One broad family of bacterial polymorphic toxins gathers multidomain proteins with a modular organization, comprising a C-terminal toxin domain fused to a N-terminal domain that adapts to the delivery apparatus. We recently described and characterized Tre23, a toxin domain fused to a T6SS-associated Rhs protein in Photorhabdus laumondii, Rhs1. Recently, we characterized a new toxin domain associated to a Rhs element in Photorhabdus laumondii. This Rhs1 toxin, encoded by the plu0353 gene, is delivered by the T6SS, through interactions with VgrG (Plu0355) and the Eag chaperone (EagR, Plu0354). Tre23 inhibits protein synthesis through ADP-ribosylation of helix 44 of the ribosomal 23 S RNA, hence preventing protein elongation by blocking the GTPase-associated center.

The Rhs1-EagR complex was purified from E. coli overproducing FLAG-tagged Rhs1 and Strep-tagged EagR by Streptag affinity followed by size-exclusion chromatography. In order to prevent Rhs1 autocleavage, a catalytic-null mutant, D1338N (see below), was used. We then performed an unmasked refinement to 3.72 Å followed by a local refinement on Rhs1Shell and obtained a resolution of 3.17 Å for this region. In the high-resolution cryo-EM densities obtained, we could build de novo an atomic model of Rhs1Shell from amino acids (aa) 272 to 1357. Rhs1Shell is composed of a continuous strip of antiparallel sheets (residues 420-1262) defining a hollow barrel, which is closed on each side by two plugs (residues 272–420 and 1263-1357 respectively). The C-terminal plug is deeply embedded in the Rhs1 β-barrel and tightly closes one side of the barrel. The N-terminal plug caps the other side of the Rhs1 β-barrel but remains at the exterior. It is composed of an Immunoglobulin-like (Ig-like) domain (336–421) preceded by a small extended domain sealing it to the Rhs1 β-barrel. The β-barrel and the two plugs define a central cavity of ~28,000 Å3 in volume. In this cavity, densities are visible but not well resolved, confirming that the C-terminal toxin domain is encapsulated into the Rhs1 β-barrel but suggesting that it is highly flexible and/or partially unfolded.

> MSLGDEIVTRIARVGARHAVHVSPPQGSPGPAAAREGDPIKHASFLGALAGAITGALIGAAVFAAASALVGLTILTGGLATVAVIALGTAATFALGDVISAASSAVTNMVDSIGPPSGTLTSGSPNVFIEGQPAARATTDIAVCSKHPAPPLIAQGSETVLINGSPAARVDDKLACGATIKSGAKTVFIGSGQGTYLAVADEFSAWERAILIAVEFLVPPSRGALKGLGKLFTKPGQGIQGVLKGAKAGAKKAKALLSNRISCAKKAFRETEGAKRYREATKKFFTGDPIDVTTGQLFDQRTDITLGQTLPLVFLRSWVPEEQGLLGPGWTDSFSECALATGDRVEIRTTEGASLYFALPAAYTHSVNPDHPDFTLSRGEQGYILRHRDSPVSKYFTLPHPSSASKEAPRRWLLTEHRDVYDNRLRFIYNKHCQLTQVLHSDGPELTLLYNLRGQLTEIRRTDERLQEVMARYHYHDNGRLAEADSTQNFHLYYEYNAQGLISRWSDGDQTWVDYRYDKQGRCTDSVGAGGFYPVHLDYAPGITRSTTPQGHTTTGHYNDQQLITEIHTPCGGVTRYEYDRWGNLVRQILPEGETLTLTYLADTGRVTSLTEATGAVWQYSYEADSLQLTGMTDPLQRTWLPQYDEQGQPAGFIAPDGRKTTLTRNAFGLVTSETDPDGNSRTQEYDKHQRLVRVLDEENRTVSLGYDSQDRLRSLTAAGALWRWRYDRHHRVAVSDRPDNQLEHFTHDRHGNLTCWTDARGVKWQVEYGPFDLPVARRDGEGHRWQYRYDADTLQLTQVINPQGETYSYTLDADGRVITEQDYAGTQWHYRYDRSGNCIEKRDGEENVTRYDYDAARRLTTLHTPEGPTRYHYDSVGRLLTVDSPDSTLHFEYDGQDRIVREIQPHGEIQRHYPDNRTAERQLLTGETAPVTGPARFSGQTHPGRWQSRREVNRVGELITLTLAGQAPLTIERDDAGRDTGRYVDGGFILRQQYSLMGQLTAQRAGRNPYFFRPAEPDEIEGPAYAGVARRYEYDTALNLTAASDDGQQVNYLLNGNGQVISVGEGRTLREHYQYDETGYPSRRFDGVQEIMGETLYQEGHRLNWVGSHRFVYDRAGRMQEKQFLAEGCRLALTKYRWNSQNQLTGLITPDGIPWEYRYDAFGRRTEKRCIQSGKLTTYLWDGNVPAEIREYQHGRLKMIRHLVFDGWELVAQQTQAFTLNLDNRVELMAGEVQTQYAVSAPTGEPLALFDPAGKRVWRRPKQSLYGLRLGGYGENPQLDPGLRFAGQLFDEESGLFYNRFRYYLPEATCYLSPDPTGLWGGENTYRYVQNPTKFINPLGLAGENVFIHATNKAGFDGIMKSGVLHPNVSGKVAITDVLMSPKDVMRDLLINNPNHIGRGDYAIIFKIDPGERGNIRSPSRLEYTHEGKLKLNNILYAGKNPYAILEHLDYDTRLKLTDNQVKIRKCGGKVDDYKDDDDK> MNKRINNNRRTMRSRRGRGRTMGSNLIPYANSPVPIPYTPPVTPVTVIGNPRKTTWIDIDLSSEESGIYTLTVG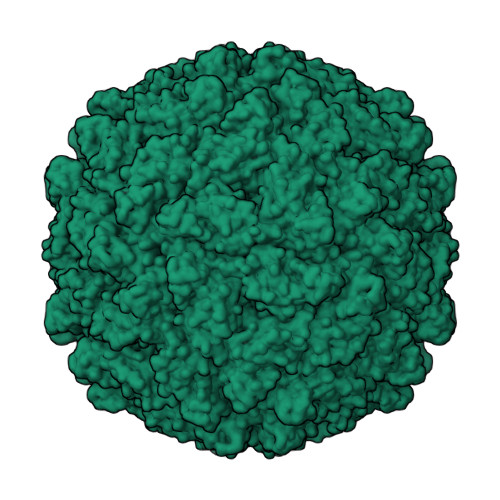SYRNRITKLGPSKPNFIIEKVAAYAAPGDYKVVLNDFKTGIQVVDEGSYAHRAAAGILYPPAAQMFYGISATGTLNTITTTAKDPVPVVRALVTYWDSEQ6-METHOXY-4-(2-{4-[([1,3]OXATHIOLO[5,4-C]PYRIDIN-6-YLMETHYL)AMINO]PIPERIDIN-1-YL}ETHYL)QUINOLINE-3-CARBONITRILE | C25 H27 N5 O2 S | 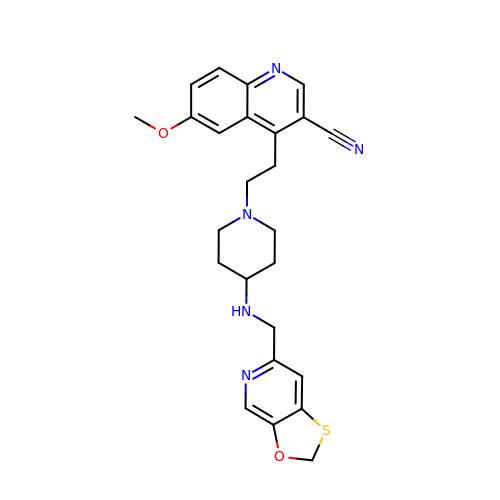NKXJSCXEAVZSMF-UHFFFAOYSA-N>[2x]GQSLELGTMQPSFTSVTGKGGVKVIDGSSVKFGRFDGAEPHCVGLTDLVTEQDGSSMAAGFMQWDNAFFPWTLNYDEIDMV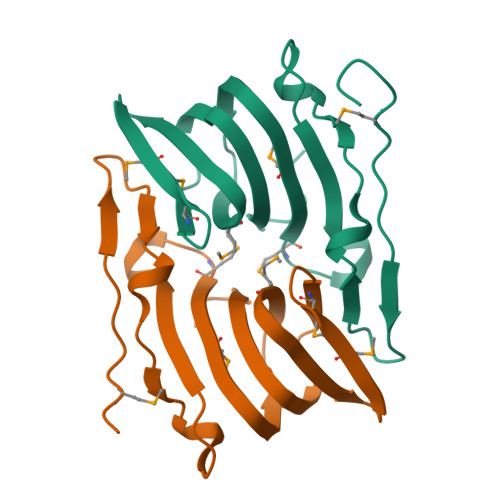LEGELHVRHEGETMIAKAGDVMFIPKGSSIEFGTPTSVRFLYVAWPANWQSV Here we describe a systematic approach to generating modular and rigid repeat protein oligomers with coincident C2 to C8 and superhelical symmetry axes that can be readily extended by repeat propagation. Repeat proteins are composed of an asymmetric structural motif that is concatenated several times in tandem within a single protein chain. From these building blocks, we demonstrate that a wide range of unbounded fibres can be systematically designed by introducing hydrophilic surface patches that force staggering of the monomers; the geometry of such fibres can be precisely tuned by varying the number of repeat units in the monomer and the placement of the hydrophilic patches. All multiplexes follow the naming convention CsHRN_Rr where s is the cyclic symmetry, HR stands for helical repeat, R is the number of repeats in a single chain and N is an index to differentiate between multiplexes of the same symmetry.

We determined the high-resolution structures of five designs from C2 to C6 symmetry by X-ray crystallography, cryogenic electron microscopy (cryoEM) or both. The crystal structure of C2HR1_4r matches the design model with an overall backbone alpha carbon (C-alpha) root mean square deviation (r.m.s.d.) of 1.54 Å. C2HR1_4r has a large repetitive interface composed primarily of leucines.

> MDYQEALLELIERLLRKLNVDPRDIKRIEQQLRDLDIYQIALLLLIILLLRKLNVDPRDIKRILQQLIDLDIYQIALLLLIILLLHKLNVDPRDIKRILQQLIDLDIEQIAELLLRILELRKRNEDPRDIKRELQQLIDDDGSWLE2-({[(2S)-1-cyclohexylpropan-2-yl]amino}methyl)phenol | C16 H25 N O | 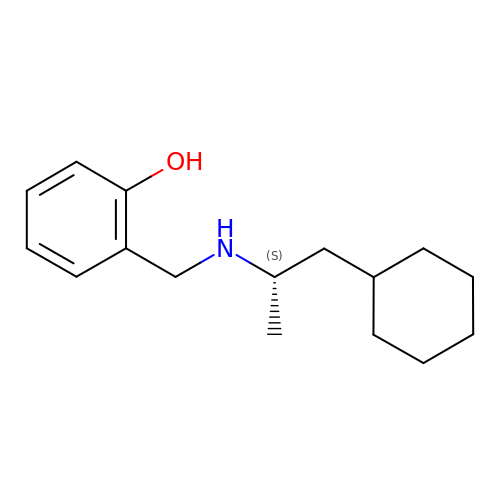IRWBEPDMVHOCPD-ZDUSSCGKSA-N1-[3-tert-butyl-1-(4-methylphenyl)-1H-pyrazol-5-yl]-3-(5-hydroxypentyl)urea 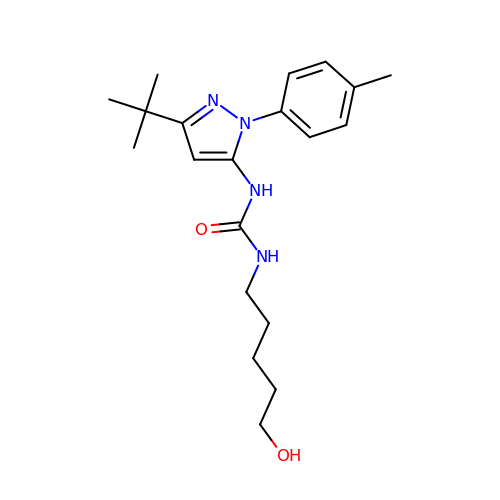| C20 H30 N4 O2 | KYUWRMMQYZFHGQ-UHFFFAOYSA-N> TTVYLAGDSTMAKNGGGSGTNGWGEYLASYLSATVVNDAVAGRSAR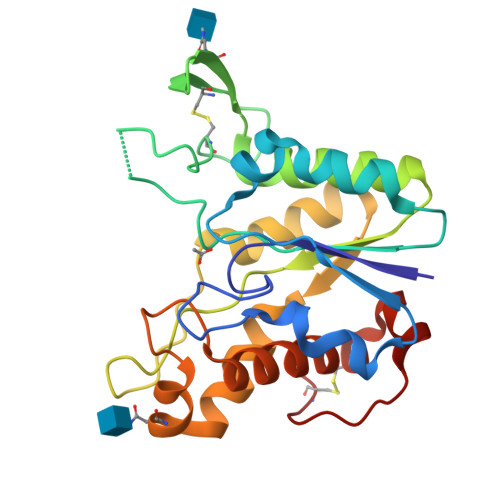SYTREGRFENIADVVTAGDYVIVEFGHNDGGSLSTDNGRTDCSGTGAEVCYSVYDGVNETILTFPAYLENAAKLFTAKGAKVILSSQTPNNPWETGTFVNSPTRFVEYAELAAEVAGVEYVDHWSYVDSIYETLGNATVNSYFPINHTHTSPAGAEVVAEAFLKAVVCTGTSLKSVLTTTSFEGTCL> MSWYPGHIEKAKRQIKDLLRLVNTVVEVRDARAPFATS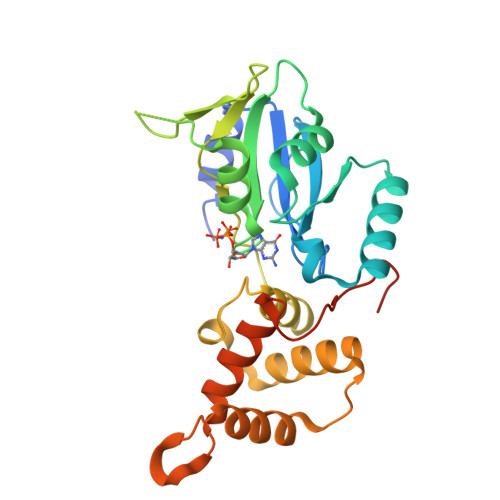AYGVDFSRKETIILLNKVDIADEKTTKKWVEFFKKQGKRVITTHKGEPRKVLLKKLSFDRLARVLIVGVPNTGKSTIINKLKGKRASSVGAQPGITKGIQWFSLENGVKILDTPGILYKNIFSEDLAAKLLLVGSLPVERIEDQRIFERAFEIFARSIGIESSFSEFFEDFARKRGLLKKGGVPDIERALMLFFTEVAQGKAGRVSFERPEDITPVQQEQTRGV> GPLGSMGNPENIEDAYVAVIRPKNTASLNSREYRAKSYEILLHEVPIEGQKKKRKKVLLETKLQGNSEITQGILDYVVETTKP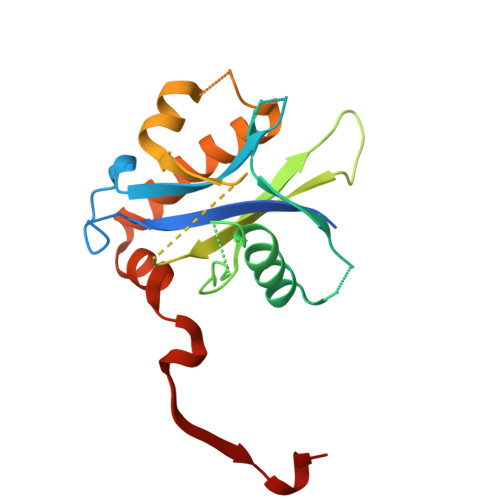ISPANQGIRGKRVVLMKKFPLDGEKMGREASLFIVPSVVKDNTKYTYTPGCPIFYCLQDIMRVCSESSTHFATLTARMLIALDKWLDERHAQSHFIPALFRPSPLERIKTNVINPAYATE BLEOMYCIN B2 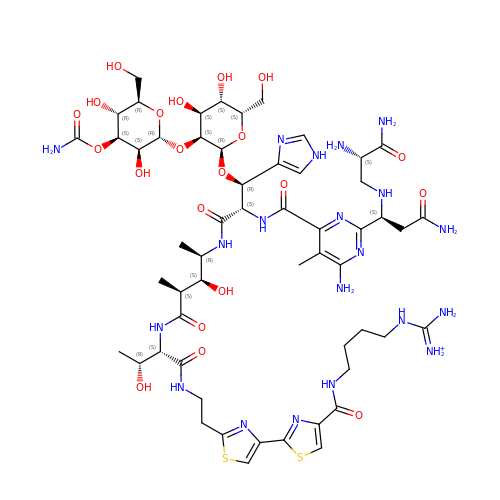| C55 H85 N20 O21 S2 | NBLHOLNNKJBEDC-XOGQCRKLSA-O>[2x]MAKAHIELTINGHPVEALVEPRTLLIHFIREQQNLTGAHIGCDTSHCGACTVDLDGMSVKSCTMFAVQANGASITTIEGMAAPDGTLSALQEGFRMMHGLQCGYCTPGMIMRSHRLLQENPSPTEAEIRFGIGGNLCRCTGYQNIVKAIQYAAAKINGVPFEEAAE;>[2x]MNIQTTVEPTSAERAEKLQGMGCKRKRVEDIRFTQGKGNYVDDVKLPGMLFGDFVRSSHAHARIKSIDTSKAKALPGVFAVLTAADLKPLNLH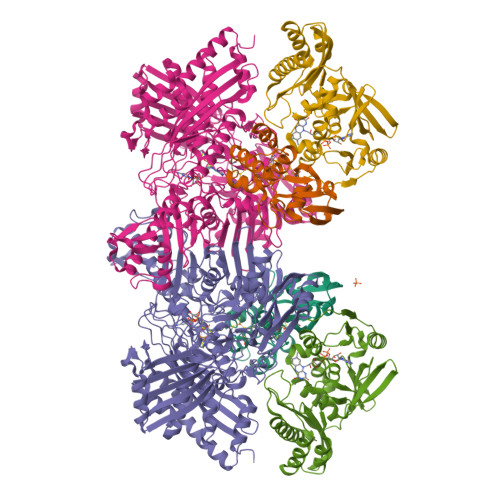YMPTLAGDVQAVLADEKVLFQNQEVAFVVAKDRYVAADAIELVEVDYEPLPVLVDPFKAMEPDAPLLREDIKDKMTGAHGARKHHNHIFRWEIGDKEGTDATFAKAEVVSKDMFTYHRVHPSPLETCQCVASMDKIKGELTLWGTFQAPHVIRTVVSLISGLPEHKIHVIAPDIGGGFGNKVGAYSGYVCAVVASIVLGVPVKWVEDRMENLSTTSFARDYHMTTELAATKDGKILAMRCHVLADHGAFDACADPSKWPAGFMNICTGSYDMPVAHLAVDGVYTNKASGGVAYRCSFRVTEAVYAIERAIETLAQRLEMDSADLRIKNFIQPEQFPYMAPLGWEYDSGNYPLAMKKAMDTVGYHQLRAEQKAKQEAFKRGETREIMGIGISFFTEIVGAGPSKNCDILGVSMFDSAEIRIHPTGSVIARMGTKSQGQGHETTYAQIIATELGIPADDIMIEEGNTDTAPYGLGTYGSRSTPTAGAATAVAARKIKAKAQMIAAHMLEVHEGDLEWDVDRFRVKGLPEKFKTMKELAWASYNSPPPNLEPGLEAVNYYDPPNMTYPFGAYFCIMDIDIDTGVAKTRRFYALDDCGTRINPMIIEGQVHGGLTEAFAVAMGQEIRYDEQGNVLGASFMDFFLPTAVETPKWETDYTVTPSPHHPIGAKGVGESPHVGGVPCFSNAVNDAYAFLNAGHIQMPHDAWRLWKVGEQLGLHV;>MIPGSFDYHRPKSIADAVALLTKLGEDARPLAGGHSLIPIMKTRLATPEHLVDLRDIGDLVGIREEGTDVVIGAMTTQHALIGSDFLAAKLPIIRETSLLIADPQIRYMGTIGGNAANGDPGNDMPALMQCLGAAYELTGPEGARIVAARDYYQGAYFTAIEPGELLTAIRIPVPPTGHGYAYEKLKRKIGDYATAAAAVVLTMSGGKCVSASIGLTNVANTPLWAEEAGKVLVGTALDKPALDKAVALAEAITAPASDGRGPAEYRTKMAGVMLRRAVERAKARAKN[2x]> EFSPAAAPPTLPPYFMKGSIIQLANGELKKVEDLKTEDFIQSAEISN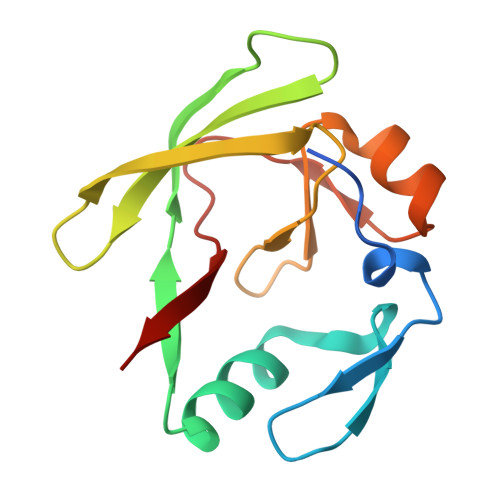DLKIDSSTVERIEDSHSPGVAVIQFAVGEHRAQVSVEVLVEYPFFVFGQGWSSCCPERTSQLFDLPCSKLSVGDVCISLTLK>MSNSDAIIYVGSFAKGTNVLMADGSIECIENIEVGNKVMGKDGRPREVIKLPRGRETMYSVVQKSQHRAHKSDSSREVPELLKFTCNATNELVVRTPRSVRRLSRTIKGVEYFEVITFEMGQKKAPDGRIVELVKEVSKSYPISEGPERANELVESYRKASNKAYFEWTIEARDLSLLGSHVRKATYQTYAPILYENDHFFDYMQKSKFHLTIEGPKVLAYLLGLWIGDGLSDRATFSVDSRDTSLMERVTEYAEKLNLCAEYKDRKEPQVAKTVNLYSKVVRGNGIRNNLNTENPLWDAIVGLGFLKDGVKNIPSFLSTDNIGTRETFLAGLIDSDGYVTDEHGIKATIKTIHTSVRDGLVSLARSLGLVVSVNAEPAKVDMNGTKHKISYAIYMSGGDVLLNVLSKCAGSKKFRPAPAAAFAR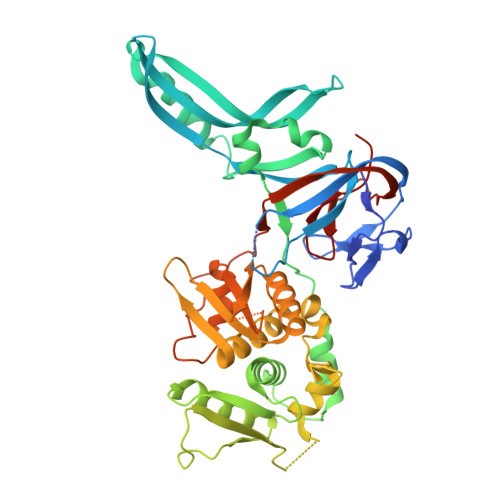ECRGFYFELQELKEDDYYGITLSDDSDHQFLLANQVVVHSSGERGNEMAE[2x]> MVVSIIPQFPDIKVSLALFEQVKNAKEIRSKMSELSTSFAFIDPRLVCSGEQMYSAIYKTLIEVKYNKMRTRNLNSECVLCLSPTSNISDAFLKFGIKDDSSQLICLKFHTNTDDVDKEQLRTIMTSIVKGQEIEFNDDNLSRFYDEALIRKIY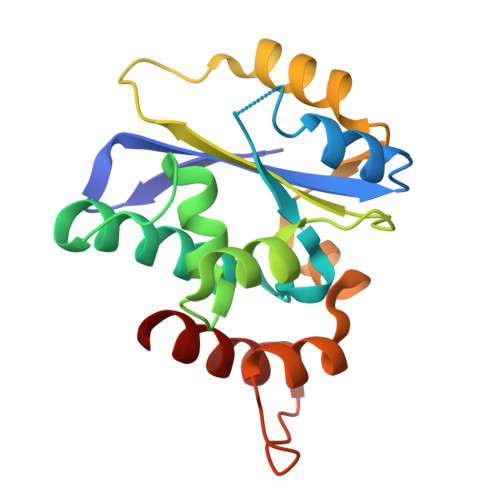KLSDDFKPQDVNGLSRALVDAIQLRGV> MSLSVEFNKQQVRPRSEISPQDCWDITPLYLNRKAWKADLDSFGLKTDGSPTWPALQATQYQLDNSESLLSLLTTLFSIERKLNKLYVYAHLTHDQDITNQEGIADLKSITHLHTLFAEETSWVQPALTSLSESLIAQHLSAPCLAPYRFYLEKIFRLSIHTGTPGEE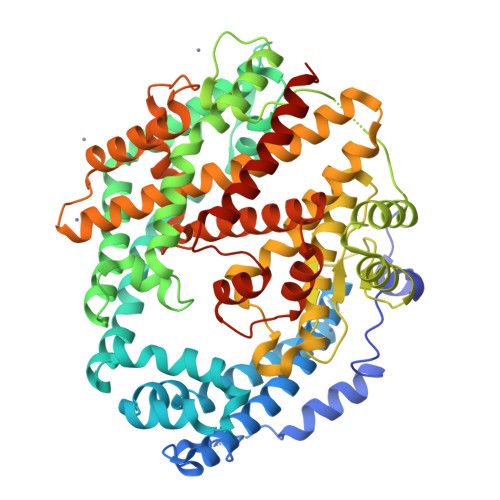KILASAFTPLEVASKAFSSLSDSEIPFGQATDSEGNSHPLSHALASLYMQSTDRELRKTSYLAQCERYHSYRHTFANLLNGKIQAHVFYAKNKRYNSCLQAALYHNNIPTTVYTNLIDIVKKNSSLITKYFSIKQRCLNLKDFHFYDVYAPLSQSKEKKYTFQEAVDLIYTSLSPLGTEYIDTLKQGLTTQGWVDKYENLNKRSGAYSSGCYDSHPYVLLNYTGTLYDVSVIAHEGGHSMHSYFSRKHQPFHDAQYPIFLAEIASTLNEMLLMDSMLKESDSKEEKITILTRCLDTIFSTLFRQVLFASFEYDIHHAAEHGVPLTEEYLSSTYKNLQNEFYGEIITFDVLSNIEWARIPHFYYNFYVYQYATGIIAALCFLEKILNNEDNALNSYLNFLKSGGSDFPLEILKKSGLDMGTVEPIQKAFCFIEKKIQELSSLIEGHHHHHH> MARKYFVAANWKCNGTLESIKSLTNSFNNLDFDPSKLDVVVFPVSVHYDHTRKLLQSKFSTGIQNVSKFGNGSCTGEVSAEIAKDLNIEYVIIGHFERRKYFHETDEDVREKLQASLKNNLKAVVCFGESLEQREQNKTIEVITKQVKAFVDLIDNFDN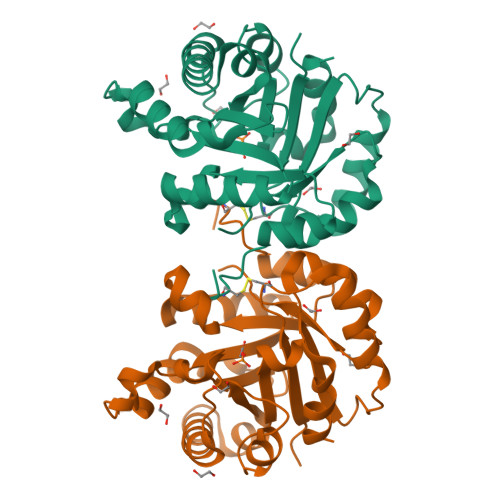VILVYEPLWAIGTGKTATPEQAQLVHKEIRKIVKDTCGEKQANQIRILYGGSVNTENCSSLIQQEDIDGFLVGNASLKESFVDIIKSAM>GLNHMTARYLREEHHMFRAAFRKFLEKEAYPHYNDWE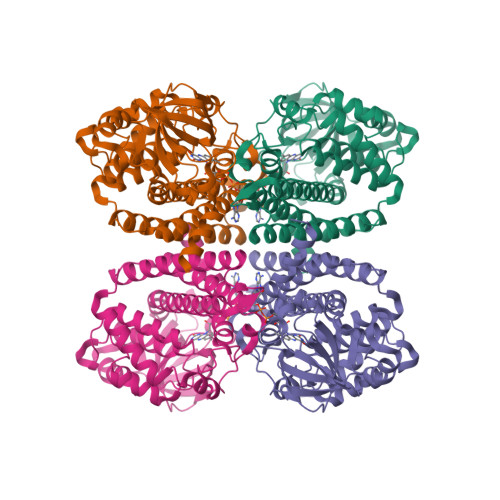KRGIIPRSFWAKMGENGFLCPWVDEKYGGLNADFAYSVVINEELEKVGSSLVGIGLHNDIVTPYIASYGTEEQKQKWLPKCVTGELITAIAMTEPGAGSDLANISTTAVKDGDYYIVNGQKTFITNGIHADLIVVACKTDPQAKPPHRGISLLVVERDTPGFTRGRKLEKVGLHAQDTAELFFQDAKVPAYNLLGEEGKGFYYLMEKLQQERLVVAIAAQTAAEVMFSLTKQYVKQRTAFGKRVSEFQTVQFRLAEMATEIALGRTFVDRVIEEHMAGKQIVTEVSMAKWWITEMAKRVAAEAMQLHGGYGYMEEYEIARRYRDIPVSAIYAGTNEMMKTIIARQLDL[2x]>CTACGCGCGTA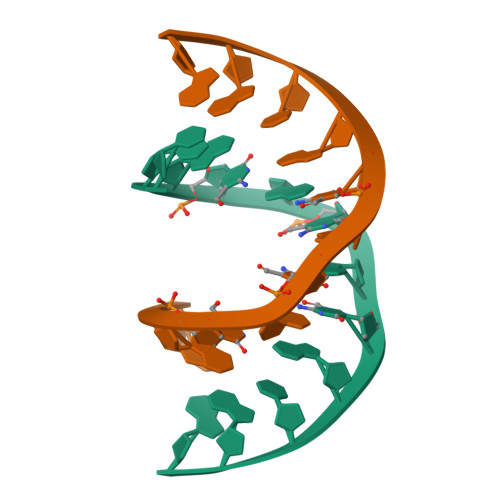G[2x]> UCCGUGAUAGUUUAAUGGUCAGAAUGGGCGCUUGUCGCGUGCCAGAUCGGGGUUCAAUUCCC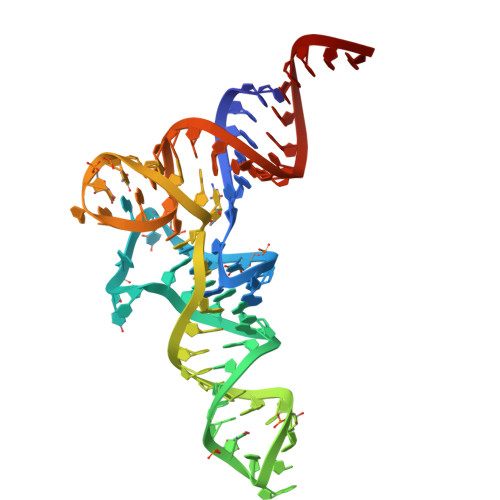CGUCGCGGAGCCA> MASDYKDDDDKLHLILLPATGNVAENSPPGTSVHKFSVKLSASLSPVIPGFPQIVNSNPLTEAFRVNWLSGTYFEVVTTGMEQLDFETGPNIFDLQIYVKDEVGVTDLQVLTVQVTDVNEPPQFQGNLAEGLHLYIVERANPGFIYQVEA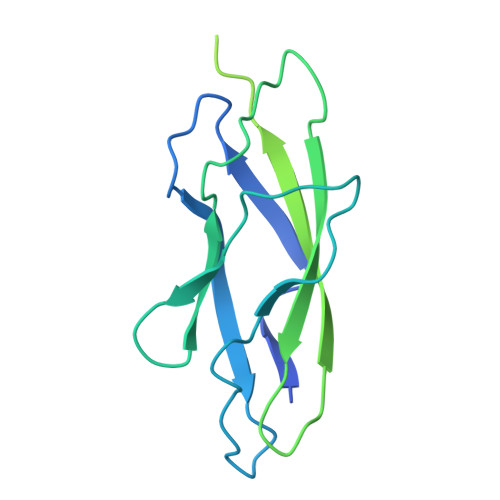FDPEDTSRNIPLSYFLISPPKSFRMSANGTLFSTTELDFEAGHRSFHLIVEVRDSGGLKASTELQVNIVNLNDEVPRFTGGTKHHHHHH>[3x]MWVRGSGPSVLSRLQDAAVVRPGFLSTAEEETLSRELEPELRRRRYEYDHWDAAIHGFRETEKS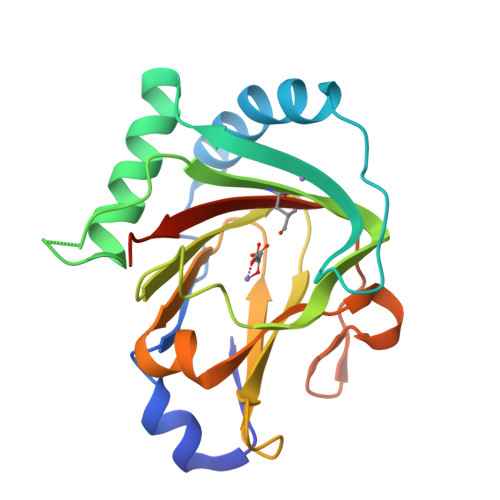RWSEASRAILRRVQAAAFGPGQTLLSSVHVLDLEARGYIKPHVDSIKFCGATIAGLSLLSPSVMRLVHTQEPGEWLELLLEPGSLYILRGSARYDFSHEILRDEESFFGERRIPRGRRISVICRSLPEGMGPGESG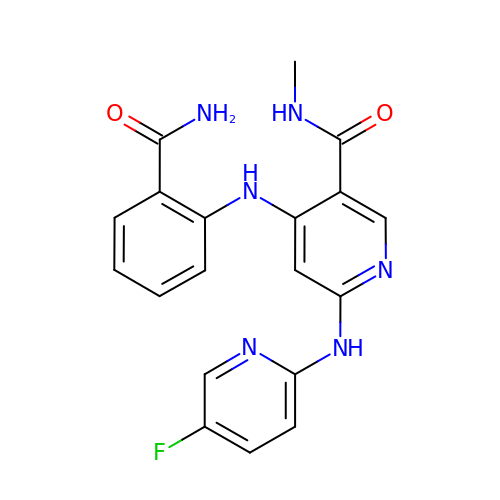4-[(2-carbamoylphenyl)amino]-6-[(5-fluoropyridin-2-yl)amino]-N-methylpyridine-3-carboxamide | C19 H17 F N6 O2 | FFYLSLMDLCQSRS-UHFFFAOYSA-N>MVSVITSEMKIELRMEGAVNGHKFVITGKGSGQPFEGIQNVDLTVIEGGPLPFAFDILTTAFHYGNRVFVEYPEEIVDYFKQSFPEGYSWERSMSYEDGGICLATNNITMKKDGSNCFVNEIRFDGVNFPANGPVMQRKTVKWEPSTEKMYVRDGVLKGDVNMALLLQGGGHYRCDFRTTYKAKKVVQLPDYHFVDHSME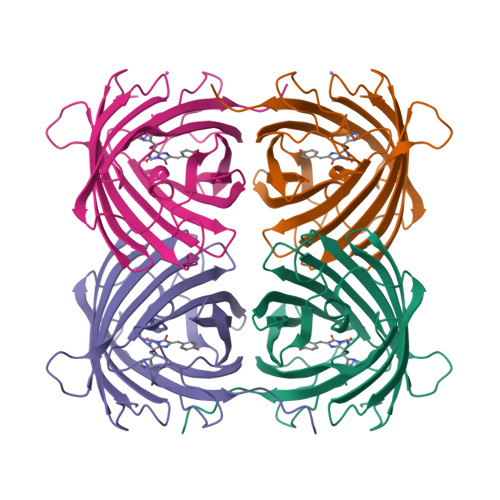ITSHDKDYNKVKLYEHAKAHSGLPRLAK[2x]> ALWQFNGMIKCKIPSSEPLLDFNN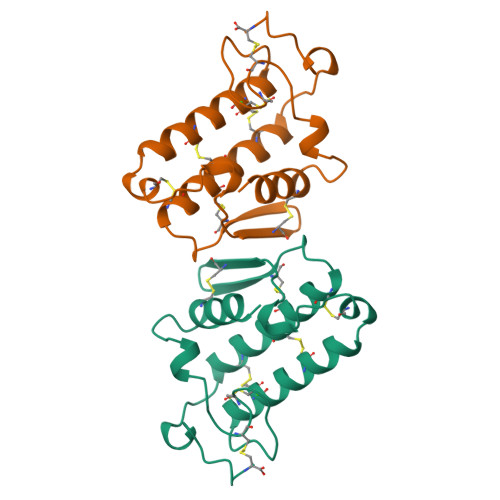YGCYCGLGGSGTPVDDLDRCCQTHDNCYKQAKKLDSCKVLVDNPYTNNYSYSCSNNEITCSSENNACEAFICNCDRNAAICFSKVPYNKEHKNLDAANC> MASEVQAERADVVIVGAGHGGAQAAIALRQNGFEGRVLVIGREPEIPYERPPLSKEYLAREKTFERICIRPAQFWEDKAVEMKLGAEVVSLDPAAHTVKLGDGSAIEYGKLIWATGGDPRRLSCVGADLAGVHAVRTKEDADRLMAELDAGAKNAVVIGGGYIGLEAAAVLTKFGVNVTLLEALPRVLARVAGEALSEFYQAEHRAHGVDLRTGAAMDCIEGDGTKVTGVRM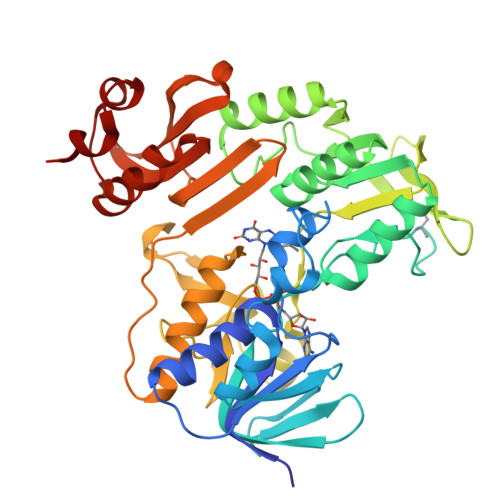QDGSVIPADIVIVGIGIVPCVGALISAGASGGNGVDVDEFCRTSLTDVYAIGDCAAHANDFADGAVIRLESVQNANDMATAAAKDICGAPVPYKATPWFWSNQYDLKLQTVGLSTGHDNAVLRGDPATRSFSVVYLKGGKVVALDCVNMVKDYVQGKKLVEARAQIAPEQLADAGVPLKEMLA>[2x]SRAPTGDPACRAAVATAQKIAPLAHGEVAALTMASAPLKLPDLAFEDADGK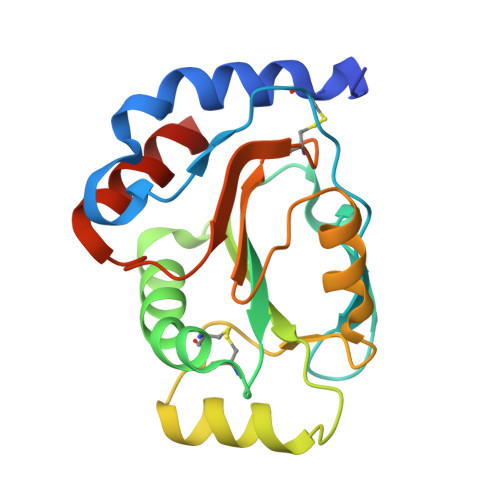PKKLSDFRGKTLLVNLWATWCVPCRKEMPALDELQGKLSGPNFEVVAINIDTRDPEKPKTFLKEANLTRLGYFNDQKAKVFQDLKAIGRALGMPTSVLVDPQGCEIATIAGPAEWASEDALKLIRAATGKAAAAL>[2x]LERGRDYEKNKVCKEFSHLGKEDFTSLSLVLYSRKFPSGTFEQVSQLVKEVVSLTEACCAEGADPDCYDTRTSALSAKSCESNSPFPVHPGTAECCTKEGLERKLCMAALKHQPQEFPTYVEPTNDEICEAFRKDPKEYANQFMWEYSTNYGQAPLSLLVSYTKSYLSMVGSCCTSASPTVCFLKERLQLKHLSLLTTLSNRVCSQYAAYGEKK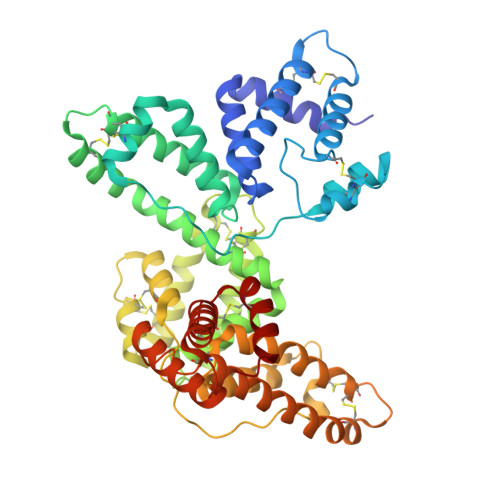SRLSNLIKLAQKVPTADLEDVLPLAEDITNILSKCCESASEDCMAKELPEHTVKLCDNLSTKNSKFEDCCQEKTAMDVFVCTYFMPAAQLPELPDVELPTNKDVCDPGNTKVMDKYTFELSRRTHLPEVFLSKVLEPTLKSLGECCDVEDSTTCFNAKGPLLKKELSSFIDKGQELCADYSENTFTEYKKKLAERLKAKLPDATPKELAKLVNKRSDFASNCCSINSPPLYCDSEIDAELKNIL> GQLLGLLGQAATVIGGEPT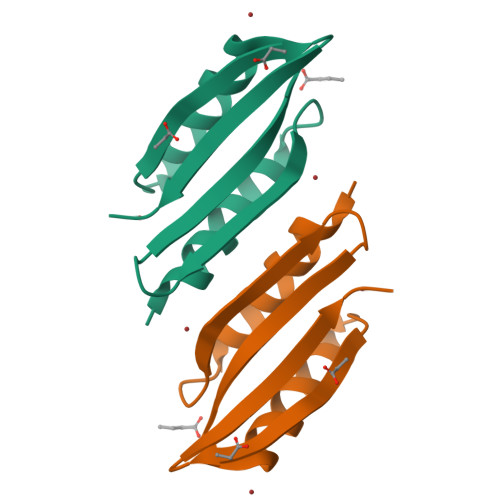VSVEQLDFSAARGDVALQVRAPGFDVLERLRSRLSESGLAVQLGSASRDGSTVSARLVIGG> RGQLQAAESRYEAQKRITQVFELEILDLYGRLEKDGLLKKLEEEK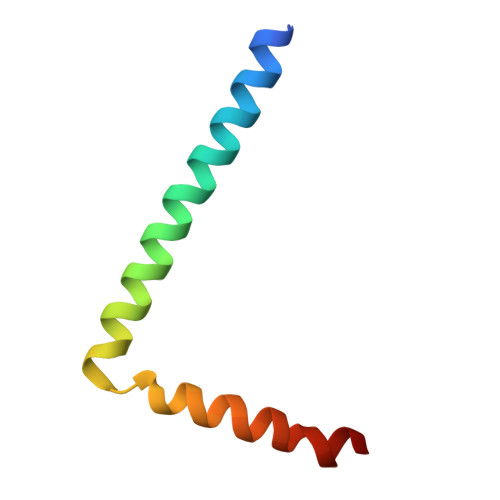AEAAEAAEERL> GPLGSLCGRVFKVGEPTYSCRDCAVDPTCVLCMECFLGSIHRDHRYRMTTSGGGGFCDCGD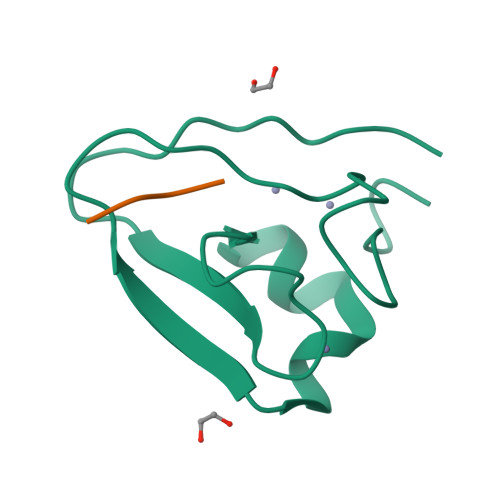TEAWKEGPYCQKHEL;> HIFS> MIIVYTTFPDWESAEKVVKTLLKERMIACANLREHRAFYWWEGKIEEDKEVGAILKTREDLWEELKE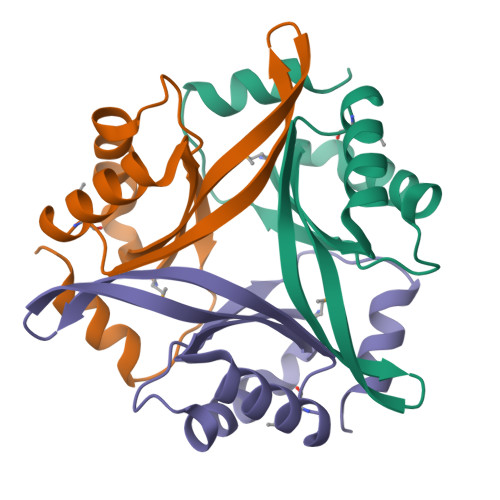RIKELHPYDVPAIIRIDVDDVNEDYLKWLIEETKK N-{(1S,2R)-2-hydroxy-1-[(hydroxyamino)carbonyl]propyl}-4-{[4-(morpholin-4-ylmethyl)phenyl]ethynyl}benzamide | C24 H27 N3 O5 | 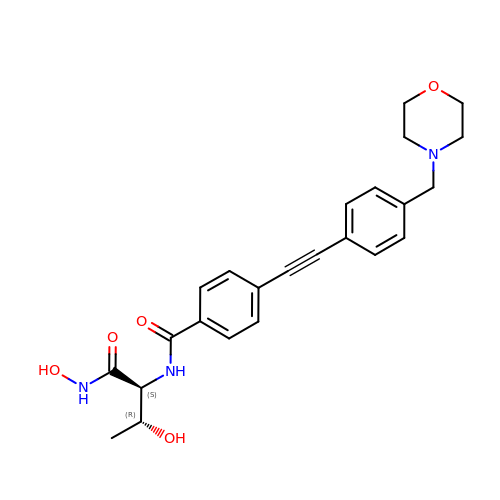FQYBTYFKOHPWQT-VGSWGCGISA-N The EphA4 tyrosine kinase cell surface receptor regulates an array of physiological processes and is the only currently known class A Eph receptor that binds both A and B class ephrins with high affinity. Eph receptors are type 1 membrane proteins with an N-terminal extracellular region consisting of a ligand binding domain (LBD), a cysteine rich region, and two fibronectin type III domains. We have solved the crystal structure of the EphA4 ligand binding domain alone and in complex with (1) ephrinB2 and (2) ephrinA2. Structural analyses, drawing on previously reported Eph receptor structures, show that EphA4 in isolation and in complex with ephrinA2 resembles other class A Eph receptors but on binding ephrinB2 assumes structural hallmarks of the class B Eph receptors. This interactive plasticity reveals EphA4 as a structural chameleon, able to adopt both A and B class Eph receptor conformations, and thus provides a molecular basis for EphA-type cross-class reactivity.

The EphA4-ephrinB2 and EphA4-ephrinA2 complex structures were solved and refined to 2.4 and 2.3 Å resolution, respectively. To facilitate crystallization of the EphA4-ephrinA2 complex, a site-directed mutation, N174Q, was incorporated into the sequence of ephrinA2 to remove a glycosylation site not conserved between ephrins. As a result, only electron density corresponding to two reducing-terminal N-acetylglucosamine residues of an N-linked sugar at Asn42ephrinA2 was observed in the EphA4-ephrinA2 structure. In contrast, the JKEphA4 loop is very different between its two bound states (2.8 Å rmsd over Cα atoms of residues Ala150EphA4-Leu166EphA4); forming an extended conformation when bound to ephrinB2 and an α helix (Gln156EphA4-Asp161EphA4) when bound to ephrinA2. The Arg162EphA4-Trp122ephrinB2 stacking interaction contrasts with that observed in the EphA4-ephrinA2 structure, where Arg162EphA4 is involved in hydrogen bonding interactions with the carbonyl oxygen of Leu138ephrinA2, while Met164EphA4and Leu166EphA4 participate in hydrophobic interactions with Leu138ephrinA2 and Phe136ephrinA2. The structural differences between the two available apo LBD structures of EphA4 and the divergence in conformational changes that occur upon ephrinB2 and ephrinA2 binding are consistent with the EphA4 receptor maintaining a high degree of structural plasticity in its DEEphA4 and JKEphA4 ephrin binding loops. These changes include the introduction of unpredicted α-helical secondary structure in the JKEphA4 loop of the EphA4-ephrinA2 complex. Based on the high degree of sequence conservation in the JK loop across all A class Eph receptors, it is likely that this α helix motif is common to all EphA-ephrinA complexes. Superposition of EphA4 and EphA2 from their ephrinA2- and ephrinA1-bound structures, respectively, reveals that the JKEph α helix is well conserved both in structure and in amino acid sequence.

> ETGEVTLLDSRSVQGELGWIASPLEGGWEEVSIMDEKNTPIRTYQVCNVMEPSQNNWLRTDWITREGAQRVYIEIKFTLRDCNSLPGVMGTCKETFNLYYYESDNDKERFIRENQFVKIDTIAADESFTQVDIGDRIMKLNTEIRDVGPLSKKGFYLAFQDVGACIALVSVRVFYKRTKHHHHHH;> ETGNSDRYAVYWNRSNPRFHAGAGDDGGGYTVEVSINDYLDIYCPHYGAPLPPAERMEHYVLYMVNGEGHASCDHRQRGFKRWECNRPAAPGGPLKFSEKFQLFTPFSLGFEFRPGHEYYYISATPPNAVDRPCLRLKVYVRPTQETLGTKHHHHHH>[2x]MKNNHLLKSILLWGAVCIIVLAGPLSAFAASSSNPSDKLYFKNKKYYIFNNVWGADQVSGWWQTIYHNSDSDMGWVWNWPSNTSTVKAYPSIVSGWHWTEGYTAGSGFPTRLSDQKNINTKVSYSISANGTYNAAYDIWLHNTNKASWDSAPTDQIMIWLNNTNAGPAGSYVETVSIGGHSWKVYKGYIDAGGGKGWNVFSFIRTANTQSANLNIRDFTNYLADSKQWLSKTKYVSS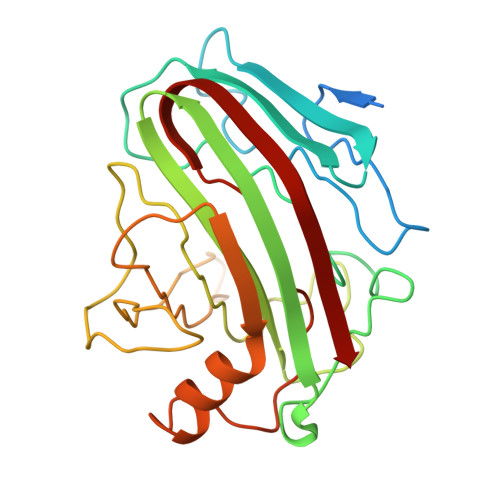VEFGTEVFGGTGQINISNWDVTVR>[2x]EHAERLPYDASKWEFPRDRLKLGKPLGRGAFGQVIEADAFGIDKTATCRTVAVKMLKEGATHSEHRALMSELKILIHIGHHLNVVNLLGACTKPGGPLMVITEFCKFGNLSTYLRSKRNEFVPYKVAPEDLYKDFLTLEHLICYSFQVAKGMEFLASRKCIHRDLAARNILLSEKNVVKICDFGLARDIYKDPDYVRKGDARLPLKWMAPETI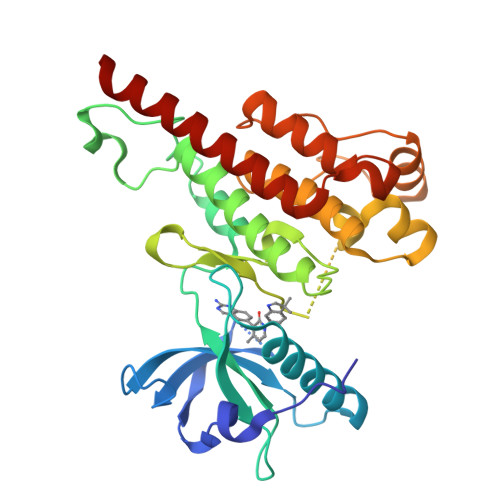FDRVYTIQSDVWSFGVLLWEIFSLGASPYPGVKIDEEFCRRLKEGTRMRAPDYTTPEMYQTMLDCWHGEPSQRPTFSELVEHLGNLLQANAQQDRHHHHHH>MSFVVIIPARYASTRLPGKPLVDINGKPMIVHVLERARESGAERIIVATD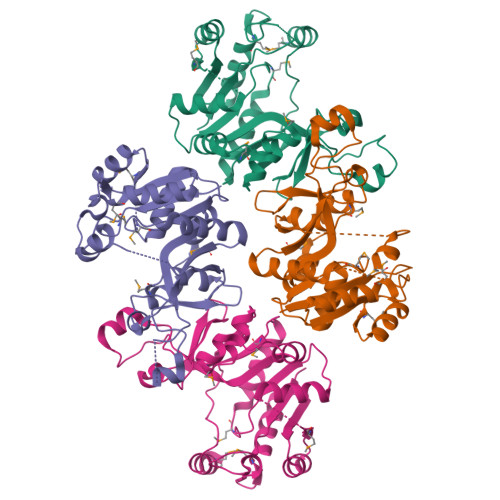HEDVARAVEAAGGEVCMTRADHQSGTERLAEVVEKCAFSDDTVIVNVQGDEPMIPATIIRQVADNLAQRQVGMATLAVPIHNAEEAFNPNAVKVVLDAEGYALYFSRATIPWDRDRFAEGLETVGDNFLRHLGIYGYRAGFIRRYVNWQPSPLEHIEMLEQLRVLWYGEKIHVAVAQEVPGTGVDTPEDLERVRAEMRGSHHHHHH[4x]N-methyl-1-(5-methyl-1,2-oxazol-3-yl)methanesulfonamide | C6 H10 N2 O3 S | 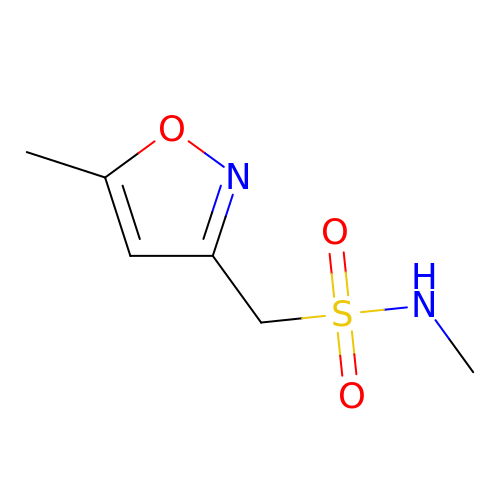SDSNLNFNGILSAL-UHFFFAOYSA-N>MKTSKTKTPKSVLIAGPCVIESLENLRSIATKLQPLANNERLDFYFKASFDKANRTSLESYRGPGLEKGLEMLQTIKEEFGYKILTDVHESYQASVAAKVADILQIPAFLCRQTDLIVEVSQTNAIVNIKKGQFMNPKDMQYSVLKALKTRDKSIQSPTYETALKNGVWLCERGSSFGYGNLVVDMRSLKIMREFAPVIFDATHSVQMPGGANGKSSGDSSFAPILARAAAAVGIDGLF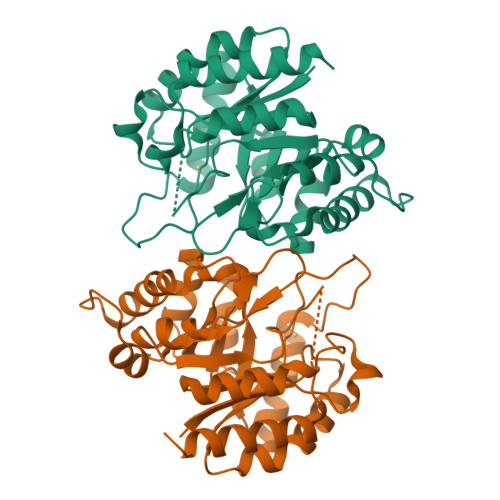AETHVDPKNALSDGANMLKPDELEQLVTDMLKIQNLF[2x]>[2x]MELYRAKFGTPERGWVVLVHGLGEHSGRYGKLIELLNGAGFGVYAFDWPGHGKSPGKRGHTSVEEAMKIIDSIIEELGEKPFLFGHSLGGLTVIRYAETRPDKIMGVVASSPALAKSPKTPSFMVALAKVLGRITPGLSLSNGLDP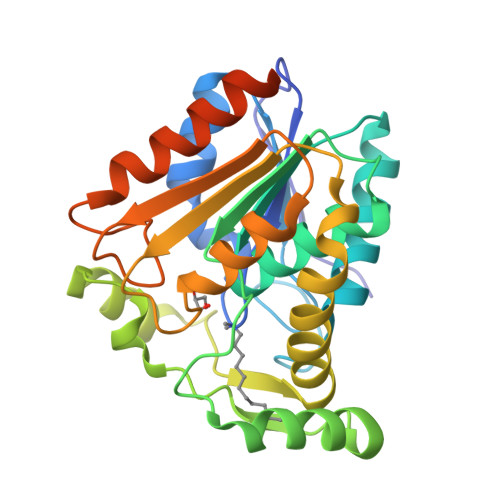KLLSRNPDAVKRYIEDPLVHDRISGKLGMSVFDNMERAHKEAERIKAPVLLLVGTADIITPPEGSRRLFEELKVKDKTIMEFKGAYHEIFEDPEWGEEFHRAIVEWLVSHSRGDLEWASAERASSIMGDSAHHHHHH> GIDPFTQNGYENPT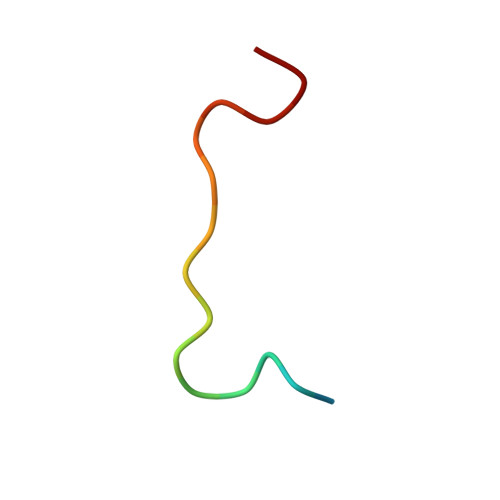YKF>AMMKAAVVRAFGAPLTIDEVPVPQPGPGQVQVKIEASGVCHTDLHAADGDWPVKPTLPFIPGHEGVGYVSAVGSGVSRVKEGDRVGVPWLYSACGYCEHCLQGWETLCEKQQNTGYSVNGGYGEYVVADPNYVGLLPDKVGFVEIAPILCAGVTVYKGLKVTDTRPGQWVVISGIGGLGHVAVQYARAMGLRVAAVDIDDAKLNLARRLGAEVAVNARDTDPAAWLQKEIGGAHGVLVTAVSPKAF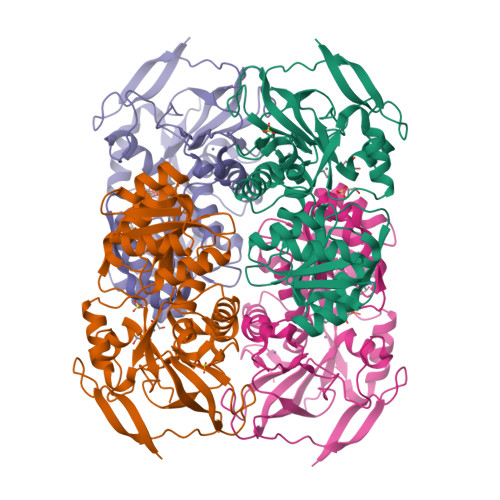SQAIGMVRRGGTIALNGLPPGDFGTPIFDVVLKGITIRGSIVGTRSDLQESLDFAAHGDVKATVSTAKLDDVNDVFGRLREGKVEGRVVLDFSR[8x]> MAQAKHKQRKRLKSSCKRHPLYVDFSDVGWNDWIVAPPGYHAFYCHGECPFPLADHLNSTNHAI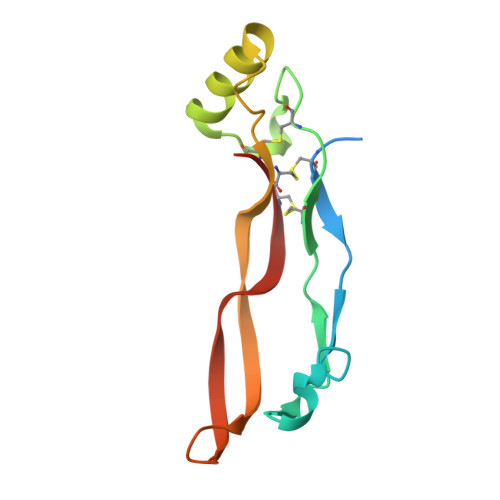VQTLVNSVNSKIPKACCVPTELSAISMLYLDENEKVVLKNYQDMVVEGCGCR> MSEFRIHHDVNELLSLLRVHGGDGAEVYIDLLQKNRTPYVTTTVSAHSAKVKIAEFSRTPEDFLKKYDELKSKNTRNLDPLVYLLSKLTEDKETLQYLQQNAKERAELAAAAVGSSTTSINVPAAASKISMQELEELRKQLGSVATGSTLQQSLELKRKMLRDKQNKKNSGQHLPIFPAWVYERPALIGDFLIGAGISTDTALPIGTLPLASQESAVVEDLLYVLVGVDGRYVSAQPLAGRQSRTFLVDPNLDLSIRELVHRILPVAASYSAVTRFIEEKSSFEYGQVNHALAAAMRTLVKEHLILVSQLEQLHRQGLLSLQKLWFYIQPAMRTMDILASLATSVDKGECLGGSTLSLLHDRSFSYTGDSQAQELCLYLTKAASAPYFEVLEKWIYRGIIHDPYSEFMVEEHELRKERIQEDYNDKYWDQRYTIVQQQIPSFLQKMADKILSTGKYLNVVRECGHDVTCPVAKEIIYTLKERAYVEQIEKAFNYASKVLLDFLMEEKELVAHLRSIKRYFLMDQGDFFVHFMDLAEEELRKPVEDITPPRLEALLELALRMSTANTDPFKDDLKIDLMPHDLITQLLRVLAIETKQEKAMAHADPTELALSGLEAFSFDYIVKWPLSLIINRKALTRYQMLFRHMFYCKHVERQLCSVWISNKTAKQHSLHSAQWFAGAFTLRQRMLNFVQNIQYYMMFEVMEPTWHILEKNLKSASNIDDVLGHHTGFLDTCLKDCMLTNPELLKVFSKLMSVCVMFTNCMQKFTQSMKLDGELGGQTLEHSTVLGLPAGAEERARKELARKHLAEHADTVQLVSGFEATINKFDKNFSAHLLDLLARLSIYSTSDCEHGMASVISRLDFNGFYTERLERLSAERSQKATPQVPVLRGPPAPAPRVAVTAQ;>[2x]MATPDQKSPNVLLQNLCCRILGRSEADVAQQFQYAVRVIGSNFAPTVERDEFLVAEKIKKELIRQRREADAALFSELHRKLHSQGVLKNKWSILYLLLSLSEDPRRQPSKVSSYATLFAQALPRDAHSTPYYYARPQTLPLSYQDRSAQSAQSSGSVGSSGISSIGLCALSGPAPAPQSLLPGQSNQAPGVGDCLRQQLGSRLAWTLTANQPSSQATTSKGVPSAVSRNMTRSRREGDTGGTMEITEAALVRDILYVFQGIDGKNIKMNNTENCYKVEGKANLSRSLRDTAVRLSELGWLHNKIRRYTDQRSLDRSFGLVGQSFCAALHQELREYYRLLSVLHSQLQLEDDQGVNLGLESSLTLRRLLVWTYDPKIRLKTLAALVDHCQGRKGGELASAVHAYTKTGDPYMRSLVQHILSLVSHPVLSFLYRWIYDGELEDTYHEFFVASDPTVKTDRLWHDKYTLRKSMIPSFMTMDQSRKVLLIGKSINFLHQVCHDQTPTTKMIAVTKSAESPQDAADLFTDLENAFQGKIDAAYFETSKYLLDVLNKKYSLLDHMQAMRRYLLLGQGDFIRHLMDLLKPELVRPATTLYQHNLTGILETAVRATNAQFDSPEILRRLDVRLLEVSPGDTGWDVFSLDYHVDGPIATVFTRECMSHYLRVFNFLWRAKRMEYILTDIRKGHMCNAKLLRNMPEFSGVLHQCHILASEMVHFIHQMQYYITFEVLECSWDELWNKVQQAQDLDHIIAAHEVFLDTIISRCLLDSDSRALLNQLRAVFDQIIELQNAQDAIYRAALEELQRRLQFEEKKKQREIEGQWGVTAAEEEEENKRIGEFKESIPKMCSQLRILTHFYQGIVQQFLVLLTTSSDESLRFLSFRLDFNEHYKAREPRLRVSLGTRGRRSSHT;>MIHELLLALSGYPGSIFTWNKRSGLQVSQDFPFLHPSETSVLNRLCRLGTDYIRFTEFIEQYTGHVQ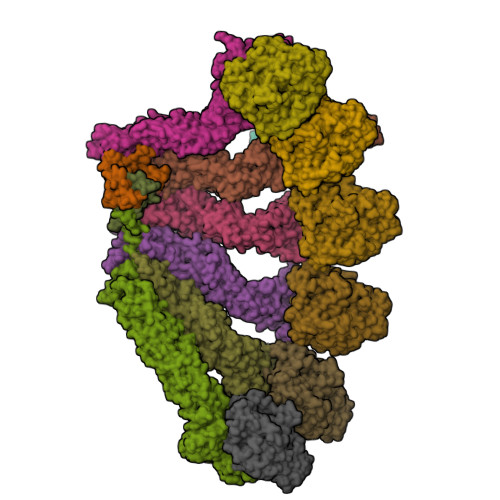QQDHHPSQQGQGGLHGIYLRAFCTGLDSVLQPYRQALLDLEQEFLGDPHLSISHVNYFLDQFQLLFPSVMVVVEQIKSQKIHGCQILETVYKHSCGGLPPVRSALEKILAVCHGVMYKQLSAWMLHGLLLDQHEEFFIKQGPSSGNVSAQPEEDEEDLGIGGLTGKQLRELQDLRLIEEENMLAPSLKQFSLRVEILPSYIPVRVAEKILFVGESVQMFENQNVNLTRKGSILKNQEDTFAAELHRLKQQPLFSLVDFEQVVDRIRSTVAEHLWKLMVEESDLLGQLKIIKDFYLLGRGELFQAFIDTAQHMLKTPPTAVTEHDVNVAFQQSAHKVLLDDDNLLPLLHLTIEYHGKEHKADATQAREGPSRETSPREAPASGWAALGLSYKVQWPLHILFTPAVLEKYNVVFKYLLSVRRVQAELQHCWALQMQRKHLKSNQTDAIKWRLRNHMAFLVDNLQYYLQVDVLESQFSQLLHQINSTRDFESIRLAHDHFLSNLLAQSFILLKPVFHCLNEILDLCHSFCSLVSQNLGPLDERGAAQLSILVKGFSRQSSLLFKILSSVRNHQINSDLAQLLLRLDYNKYYTQAGGTLGSFGM[2x];>[2x]MARHGPPWSRLDAQQERDVRELVRGVAGLQDEADPNFQLALNFAWSNFRFHRFLDVNSHKIEKTIEGIYEKFVIHSDLSKAASWKRLTEEFLNAPLPSIKEIKTDAHYSILSLLLCLSDSPSNSSYVETPRNKEVEKKDDFDWGKYLMEDEEMDIGPYMDTPNWSEESEEENDQQPLSREDSGIQVDRTPLEEQDQNRKLDPCISWKDEPDDRSWLEHHVVHQYWTARPSQFPHSLHLHSNLAAVWDQHLYSSDPLYVPDDRVLVTETQVIRETLWLLSGVKKLFIFQLIDGKVTVRNNIIVTHLTHSCLRSVLEQIAAYGQVVFRLQEFIDEVMGHSSESMLPGSGSVPKKSTEAPFRTYQAFMWALYKYFISFKEELAEIEKCIINNDTTITLAIVVDKLAPRLSQLKVLHKVFSTGVAEVPPDTRNVVRASHLLNTLYKAILEYDNVGEASEQTVSLLFSLWVETVRPYLQTVDEWIVHGHLWDGAREFIIQRNKNVPVNHRDFWYATYTLYSVSEKTENEEKMSDNASASSGSDQGPSSRQHTMVSFLKPVLKQIIMAGKSMQLLKNLQCAESTTCQAGARDAERKSLYTLFLESVQSRLRHGEDSTPQVLTEQQATKENLMKMQSIAESHLELDDVHDPLLAINFARMYLEQSDFHEKFAGGDVCVDRSSESVTCQTFELTLRSCLYPHIDKQYLDCCGNLMQTLKKDYRLVEYLQAMRNFFLMEGGDTMYDFYTSIFDKIREKETWQNVSFLNVQLQEAVGQRYPEDSSRLSISFENVDTAKKKLPVHILDGLTLSYKVPWPVDIVISLECQKIYNQVFLLLLQIKWAKYSLDVLLFGELVSTAEKPRLKEGLIHEQDTVAQFGPQKEPVRQQIHRMFLLRVKLMHFVNSLHNYIMTRILHSTGLEFQHQVEEAKDLDQLIKIHYRYLSTIHDRCLLREKVSFVKEAIMKVLNLALMFADGWQAGLGTWRMESIEKMESDFKNCHMFLVTILNKAVCRGSFPHLESLALSLMAGMEQS;> MASITQLFDDLCEALLPAAKTHLGQRSVNRKRAKRSLKKVAYNALFTNLFQDETQQLQPDMSKLPARNKILMLSFDLRVGGLGPKADRLEELVEELEAAPCCPLLEVGSVLDLLVQLAGSGPPQVLPRKRDYFLNNKHVGRNVPYSGYDCDDLSVFEMDVQSLISREECLCHSMIQETLQVMEAAPGTGLPTVGLFSFGDPCGDRFERDTRVSLFGALVHSRTYDMDVRLGLPPVPDNADLSGLAIKVPPSVDQWEDEGFQSASNLTPDSQSEPSVTPDVDLWEAALTYEASKRRCWERVGCPPGHREEPYLTEAGRDAFDKFCRLHQGELQLLAGGVLQAPQPVLVKECELVKDVLNVLIGVVSATFSLCQPAQAFVVKRGVHVSGASPESISSLLSEVAEYGTCYTRLSHFSLQPVLDSLYSKGLVFQAFTSGLRRYLQYYRACVLSTPPTLSLLTIGFLFKKLGRQLRYLAELCGVGAVLPGTCGGGPRAAFPTGVKLLSYLYQEALHNCSNEHYPVLLSLLKTSCEPYTRFIHDWVYSGVFRDAYGEFMIQVNHEYLSFRDKLYWTHGYVLISKEVEDCVPVFLKHIAHDIYVCGKTINLLKLCCPRHYLCWSDVPVPRISVIFSLEELKEIEKDCAVYVGRMERVARHSSVSKEEKELRMEIAKQELIAHAREAASRVLSALSDRQMSERMALDARKREQFQRLKEQFVKDQERRQAARQEELDDDFSYARELRDRERRLKSLEEELERKARQALVDHYSKLSAEAARREQKALWRIQRHRLESARLRFLLEDEKHIQEMLKAVSEAHQPQEPPDVLLSVHPQVTSPGPEHPEGGQGCDSGSAEQHSPAWDGWNRPGLLTPQPLKPLAVGAGGRGLQQAEGARPFSDSLSIGDFLPVGPGAEPSVQTGMVPLLEVALQTINLDLPPSAPGEAPAAASTQPSRPQEYDFSTVLRPAVATSPAPGPLQAAECSLGSSGLQLWEDSCGKMDACGSASRETLLPSHPPRRAALEEGSSQPTERLFGQVSGGGLPTGDYASEIAPTRPRWNTHGHVSDASIRVGENVSDVAPTQPRWNTHGHVSNASISLGESVSDVAPTRPRWNIHGHVSNASIRVGENVSDVAPTRPRWNTHGHVSNASIRVGENVSDVAPTRPRWNTHGHVSDASISLGESVSDMAPARPRWNTHGHVSDASISLGESVSDMAPTRPRWNTHGHVSDTSIRVGENVSDVAPIRSRCNTHGHVSDASISLGEPVSDVVSTRPRWNTHVPIPPPHMVLGALSPEAEPNTPRPQQSPPGHTSQSALSLGAQSTVLDCGPRLPVEVGPSLSSPSSGCGEGSISVGENVSDVAPTQPWWPNTPGDSVSEELGPGRSGDTEDLSPNWPLNSQEDTAAQSSPGRGEEAEASAAEAQGGEQAYLAGLAGQYHLERYPDSYESMSEPPIAHLLRPVLPRAFAFPVDPQVQSAADETAVQLSELLTLPVLMKRSITAPLAAHISLVNKAAVDYFFVELHLEAHYEALRHFLLMEDGEFAQSLSDLLFEKLGAGQTPGELLNPLVLNSVLSKALQCSLHGDTPHASNLSLALKYLPEVFAPNAPDVLSCLELRYKVDWPLNIVITEGCVSKYSGVFSFLLQLKLMMWALKDVCFHLKRTALLSHMAGSVQFRQLQLFKHEMQHFVKVIQGYIANQILHVTWCEFRARLATVGDLEEIQRAHAEYLHKAVFRGLLTEKAAPVMNVIHSIFSLVLKFRSQLISQAWGPPGGPRGAEHPNFALMQQSYNTFKYYSHFLFKVVTKLVNRGYQPHLEDFLLRINFNNYYQDA;>[6x]MPREIITLQLGQCGNQIGFEFWKQLCAEHGISPEGIVEEFATEGTDRKDVFFYQADDEHYIPRAVLLDLEPRVIHSILNSPYAKLYNPENIYLSEHGGGAGNNWASGFSQGEKIHEDIFDIIDREADGSDSLEGFVLCHSIAGGTGSGLGSYLLERLNDRYPKKLVQTYSVFPNQDEMSDVVVQPYNSLLTLKRLTQNADCVVVLDNTALNRIATDRLHIQNPSFSQINQLVSTIMSASTTTLRYPGYMNNDLIGLIASLIPTPRLHFLMTGYTPLTTDQSVASVRKTTVLDVMRRLLQPKNVMVSTGRDRQTNHCYIAILNIIQGEVDPTQVHKSLQRIRERKLANFIPWGPASIQVALSRKSPYLPSAHRVSGLMMANHTSISSLFERTCRQYDKLRKREAFLEQFRKEDMFKDNFDEMDTSREIVQQLIDEYHAATRPDYISWGTQEQ;>[2x]MASSSGAGAAAAAAAANLNAVRETMDVLLEISRILNTGLDMETLSICVRLCEQGINPEALSSVIKELRKATEALKAAENMTS2,4-DINITROPHENOL | C6 H4 N2 O5 | 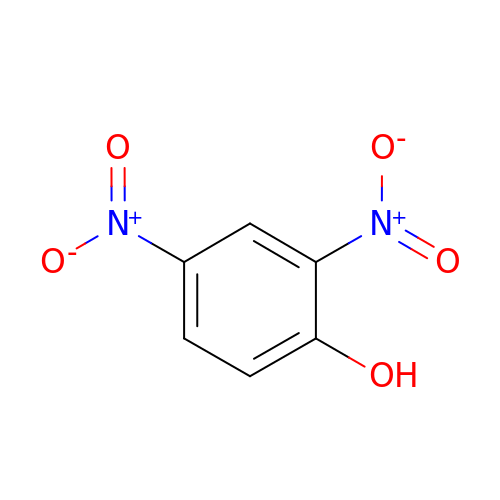UFBJCMHMOXMLKC-UHFFFAOYSA-N>[8x]MAHHHHHHAALRQPQVAELLAEARRAFREEFGAEPELAVSAPGRVNLIGEHTDYNQGLVLPMALELMTVLVGSPRKDGLVSLLTTSEGADEPQRLQFPLPTAQRSLEPGTPRWANYVKGVIQYYPAAPLPGFSAVVVSSVPLGGGLSSSASLEVATYTFLQQLCPDSGTIAARAQVCQQAEHSFAGMPCGIMDQFISLMGQKGHALLIDCRSLETSLVPLSDPKLAVLITNSNVRHSLASSEYPVRRRQCEEVARALGAASLREVQLEELEAARDLVSKEGFRRARHVVGEIRRTAQAAAALRRGDYRAFGRLMVESHRSLRDDYEVSCPELDQLVEAALAVPGVYGSRMTGGGFGGCTVTLLEASAAPHAMRHIQEHYGGTATFYLSQAADGAKVLCL

GALK1 is a small molecule kinase of the GHMP kinase family, which catalyzes the MgATP-dependent phosphorylation of the C-1 hydroxyl of α-d-galactose to yield Gal-1-P in the Leloir pathway. In classic galactosemia, GALT enzymatic deficiency causes the accumulation of Gal-1-P, the product of the enzyme galactokinase 1 (GALK1; EC 2.7.1.6) upstream of GALT in the Leloir pathway. Inhibition of human GALK1 (hGALK1) to prevent Gal-1-P production therefore could provide a therapeutic benefit for GALT deficiency. Here, we determined crystal structures of hGALK1 bound with reported ATP-competitive inhibitors of the spiro-benzoxazole series, to reveal their binding mode in the active site.

To this end, we co-crystallized hGALK1 with two spiro-benzoxazole inhibitors (T1 and T2), in the presence of galactose, and determined their crystal structures to 2.44 and 2.10 Å resolution, respectively. T1 and T2 share the chemical scaffold of a benzoxazole ring connected to a tetrahydroquinazolinone ring by an amide linker, and both compounds are found to occupy the ATP binding site in a similar manner. The benzoxazole ring, mimicking the adenine moiety of ATP, sits in a hydrophobic pocket forming a π–π stacking interaction with Trp106 and van der Waals interactions with Val129 and Leu145. The amide linker and dihydropyrimidine substituent of the quinazolinone ring occupy a similar position to that of the ATP ribose moiety. Both compounds elicit changes in the four active site loops involved in ATP binding. Importantly, the quinazolinone cyclohexanone and spiro-ring substituents cause displacement of two key side-chains—Arg105 and Arg228—at the entrance of the ATP site. In our costructures, both Arg105 and Arg228 are sequestered away from the ATP phosphate groups, to accommodate the quinazolinone ring of the compounds. Therefore, these residues are sequestered away from catalysis in the inhibitor-bound complexes. We observed dose-dependent inhibition of hGALK1, with IC50’s (T1: IC50 12 μM, pIC50 4.9 ± 0.2; T2: IC50 17 μM, pIC50 4.8 ± 0.1) similar to published values.>[2x]MENFPTEYFLNTTVRLLEYIRYRDSNYTREERIENLHYAYNKAAHHFAQPRQQQLLKVDPKRLQASLQTIVGMVVYSWAKVSKECMADLSIHYTYTLVLDDSKDDPYPTMVNYFDDLQAGREQAHPWWALVNEHFPNVLRHFGPFCSLNLIRSTLDFFEGCWIEQYNFGGFPGSHDYPQFLRRMNGLGHCVGASLWP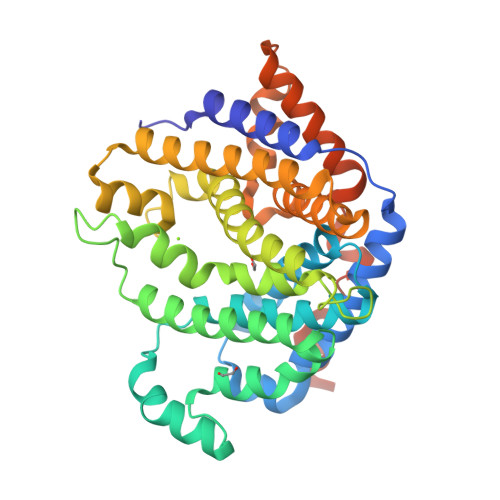KEQFNERSLFLEITSAIAQMENWMVWVNDLMSFYKEFDDERDQISLVKNYVVSDEISLHEALEKLTQDTLHSSKQMVAVFSDKDPQVMDTIECFMHGYVTWHLCDRKYRLSEIYEKVKEEKTEDAQKFCKFYEQAANVGAVSPSEWAYPPVAQLANVRSKDVKEVQKPFLSSIELVE> GGCGCGAGGAAGGAG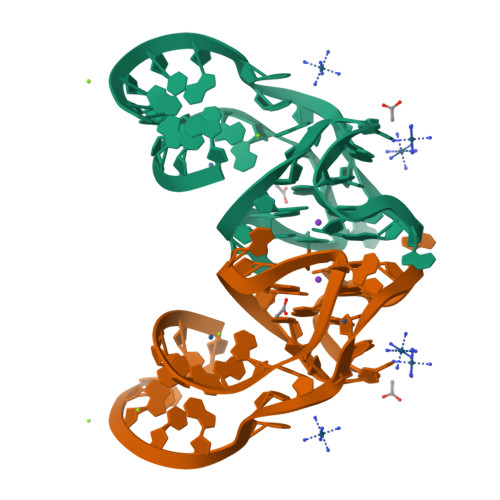GUCUGAGGAGGUCACUGCGCC>MVRVTTNPVDLWSAPSSQARLEKEYFDQHFGPFFRTEQLIIRAPLTDKHIYQPYPSGADVPFGPPLDIQILHQVLDLQIAIENITASYDNETVTLQDICLAPLSPYNTNCTILSVLNYFQNSHSVLDHKKGDDFFVYADYHTHFLYCVRA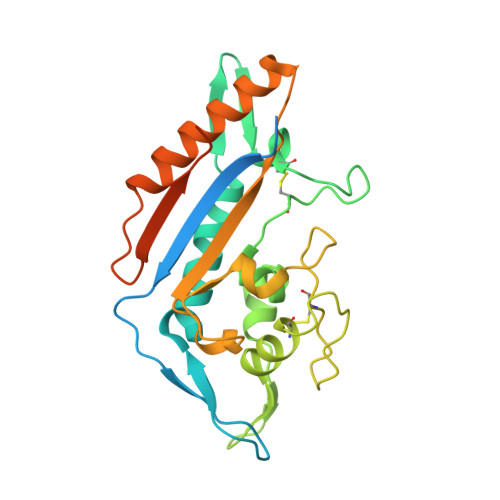PASLNDTSLLHDPCLGTFGGPVFPWLVLGGYDDQNYNNATALVITFPVNNYYNDTEKLQRAQAWEKEFINFVKNYKNPNLTISFTAERSIEDELNRESDSDVLEHHHHHHHH[2x]Herein we provide evidence that Ca2+- and redox-dependent regulation is directly linked within one protein, involved in the regulation of photosynthetic redox regulation and oxidative stress defense. This protein is designated as calredoxin (CRX, Cre03.g202950.t1.1) and consists of 4 EF-hands that are functionally connected to a TRX domain. In this work we characterized functional properties of CRX, which is conserved in the green algae lineage but absent in vascular plants. Therefore, we conclude that CRX is localized in the chloroplast stroma of Chlamydomonas. In this work we characterized a protein designated as CRX, representing a new class of Ca2+-dependent ‘sensor-responder' proteins.

The phases of the native crystal data were obtained by the molecular replacement method and the structure was refined to 1.6 Å resolution. The crystal contained two CRX molecules per asymmetric unit and the electron density map was clear enough to refine the model without any non-crystallographic restraint. Molecules A and B contained 313 and 310 amino acid residues, respectively, except for flexible regions, four calcium ions in each CRX molecule and 1,156 water molecules in total. The CRX molecule consists of two domains connected by a flexible linker region: the CaM domain with four Ca2+-binding EF-hand loops and the TRX domain with one disulfide bridge. In the CaM domain, one calcium ion was bound in each EF-hand loop located in the N- and C-subdomains, respectively. The TRX domain exhibited the typical TRX fold, possessing four α-helices (H10–H13) and one mixed β-sheet. Side chains of Cys238 and Cys241 formed the disulfide bridge between the second β-strand and the H11 helix. At the interface of the two domains, extensive inter-domain interactions were found. There were two hydrogen bond networks between the active site of the TRX domain and the Ca4 binding site. However, it appears that the TRX activity of CRX needs Ca2+, as the TRX domain without the CaM domain is functionally inactive. This is an intriguing aspect as the structure of the TRX domain showed noteworthy similarity to the conventional TRX molecule (r.m.s.d=1.36 Å for Cα atoms of spinach TRX f), strongly suggesting that the Ca2+-dependent activity of CRX is modulated via the inter-domain communication path which is absent in TRX f.

>MCSARSVRVVPRAATFEGLMDDASKAKMEELERRFKMADVDGNGHIDREELRNLLESMESGEVYMMSQHWLPEDELERCMEQYDVNKDGVISFEEFKQIIYDGLLLEGTLAEYESAFKAVDKSGNGTIGATELSKLFASLGNPVSLEKLVDLMQMYDKDDSGQIEFPEFLLMFRNSLLDLKDMTTYMTLDEAGAGSSGSLVDAVEGDMTLIFSEEELDALISANPDKLVVVFGALTWCRPCKGMQRPVQKLAEHYKDHIVFVKLFGNANKQTKRIFKERFQIRSTPCFITLRKGEPVYTQTGSNKEKLEAGLRSLIANPPVGMIYPSAEALAALQDPNSSSVDKLAAALEHHHHHH[2x]> GGGHNVAWDYDNNVIRGVNLGGWFVLEPYMTPSLFEPFQNGNDQSGVPVDEYHWTQTLGKEAALRILQKHWSTWITEQDFKQISNLGLNFVRIPIGYWAFQLLDNDPYVQGQVQYLEKALGWARKNNIRVWIDLHGAPGSQNGFDNSGLRDSYNFQNGDNTQVTLNVLNTIFKKYGGNEYSDVVIGIELLNEPLGPVLNMDKLKQFFLDGYNSLRQTGSVTPVIIHDAFQVFGYWNNFLTVAEGQWNVVVDHHHYQVISGGELSRNINDHISVACNWGWDAKKESHWNVAGEWSAALTDC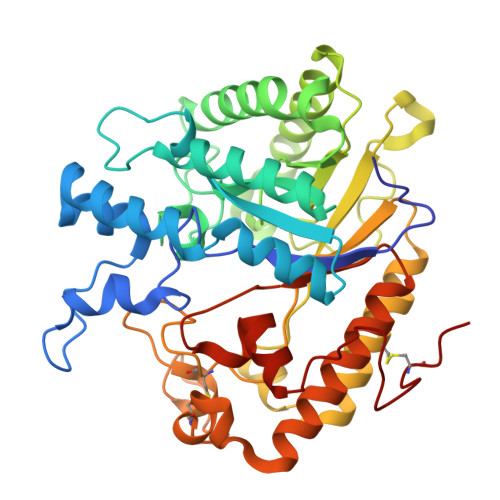AKWLNGVNRGARYEGAYDNAPYIGSCQPLLDISQWSDEHKTDTRRYIEAQLDAFEYTGGWVFWSWKTENAPEWSFQTLTYNGLFPQPVTDRQFPNQCGFH>[2x]MIQMVKRVHIFDWHKEHARKIEEFAGWEMPIWYSSIKEEHLAVRNAVGIFDVSHM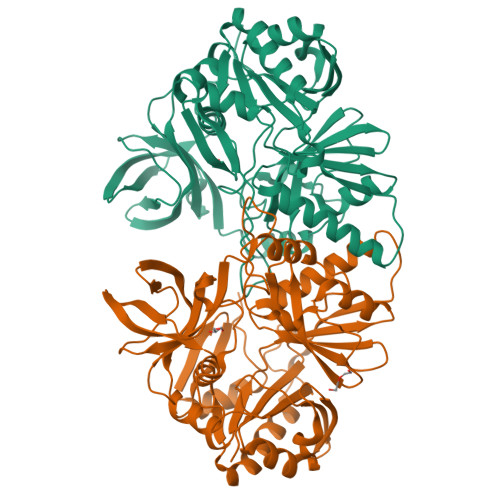GEIVFRGKDALKFLQYVTTNDISKPPAISGTYTLVLNERGAIKDETLVFNMGNNEYLMICDSDAFEKLYAWFTYLKRTIEQFTKLDLEIELKTYDIAMFAVQGPKARDLAKDLFGIDINEMWWFQARWVELDGIKMLLSRSGYTGENGFEVYIEDANPYHPDESKRGEPEKALHVWERILEEGKKYGIKPCGLGARDTLRLEAGYTLYGNETKELQLLSTDIDEVTPLQANLEFAIYWDKDFIGKDALLKQKERGVGRKLVHFKMIDKGIPREGYKVYANGEMIGEVTSGTLSPLLNVGIGIAFVKEEYAKPGIEIEVEIRGQRKKAVTVTPPFYDPKKYGLFRET> GDRVADMIESSIGNSVSRALTQALPAPTGQNTQVSSHRLDTGEVP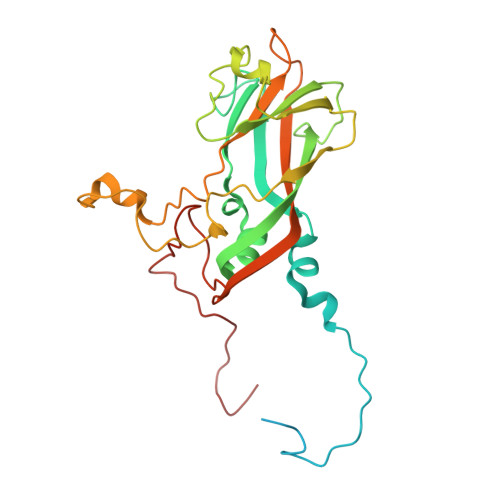ALQAAEIGASSNTSDESMIETRCVLNSHSTAETTLDSFFSRAGLVGEIDLPLEGTTNPNGYANWDIDITGCAQMRRKVELFTYMRFDAEFTFVACTPTGQVVPQLLQYMFVPPGAPIPESRESLAWQTATNPSVFVKLTDPPAQVSVPFMSPASAYQWFYDGYPTFGEHKQEKDLEYGACPNNMMGTFSVRTVGSSKSKYALVVRIYMRMKHVRAWIPRPMRNQNYLFKANPNYAGDSIKPTGTSRNAITTL In this paper, we describe the molecular architecture of the prototypical bacterial SNARE-like protein IncA, which mediates the homotypic fusion of chlamydial inclusions. IncA is a protein of 273 amino acids composed of a short, cytoplasmic N-terminal moiety (residues 1–34), a bilobed transmembrane domain (residues 35–84), and a long cytoplasmic C-terminal domain that ends in a tail with low complexity (residues 247–273). We demonstrate that IncA folds into a stable, non-canonical four-helix bundle that is maintained as a monomer by intramolecular interactions. Cells infected with an IncA-deficient strain of C. trachomatis similarly displayed multiple inclusions at a high multiplicity of infection, further establishing that IncA is required for the homotypic fusion of inclusions.

To characterize these regions, we first generated a G144A hinge mutant variant and found that IncA87–246(G144A) remains monomeric in solution and it has comparable structural stability as IncA87–246. IncA87–246(G144A) crystallized in a triclinic space group with two IncA87–246(G144A) protomers in the unit cell. Though this crystal form did not diffract as well as the previous one, we were able to collect 88.1% complete data to 1.95 Å resolution and determine an accurate atomic model of IncA87–246(G144A) using molecular replacement. The structure, solved to a Rwork/free of 16.9/21.2 at 1.95 Å resolution, contains two four-helix bundles where the interrupted α-helix HB of IncA87–246 is replaced by a straight continuous helix. Interestingly, the two IncA87–246(G144A) protomers in the triclinic unit cell are noticeably dissimilar (RMSD 1.65 Å), with protomer B characterized by a local unfolding of helix A between residues 100VGSL103. In both protomers, this region is not implicated in crystal contacts, which suggests IncA87–246(G144A) may exist in solution in different microstates, also populated in the crystal lattice. Secondary structure superimposition of IncA87–246 with the reference IncA87–246(G144A) protomer A reveals the G144A mutation results in significant conformational changes throughout the molecule (RMSD 1.68 Å), especially in the helix HD, which is shifted upwards in IncA87–246(G144A). Simulation of IncA87–246(G144A) revealed a spike in RMSF at residue 231, a feature which is absent in both the IncA87–246 and IncA87–237 RMSF profiles. This result agrees with the structural plasticity of IncA87–246(G144A) protomers seen in the triclinic crystal form, which deviate significantly at the C-terminus of helix HD. However, when G144 of the hinge is mutated to alanine, the HD–Hclamp distance narrows and results in a significantly less flexible Hclamp during simulation compared with IncA87–246 and IncA87–237, which may explain experimental results regarding the lack of IncA87–246(G144A) oligomerization in solution.

>ATANLHLYQDLQREVGSLKEINFMLSVLQKEFLHLSKEFATTSKDLSAVSQDFYSCLQAFRDNYKGFESLLDEYKNSTEEMRKLFSQEIIADLKGSVASLREEIRFLTPLAEEVRRLAHNQQSLTAAIEELKTIRDSLRDEIGQLSQLSKTLTSQIALQRKLEHHHHHH[2x]> HMEEMIRSLQQ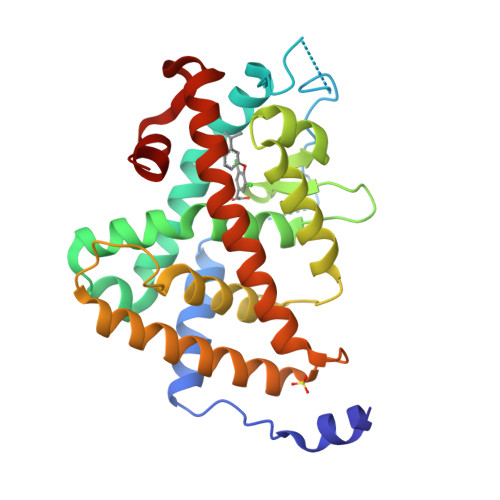RPEPTPEEWDLIHIATEAHRSTNAQGSHWKQRRKFLPDDIGQSPIVSMPDGDKVDLEAFSEFTKIITPAITRVVDFAKKLPMFSELPCEDQIILLKGCCMEIMSLRAAVRYDPESDTLTLSGEMAVKREQLKNGGLGVVSDAIFELGKSLSAFNLDDTEVALLQAVLLMSTDRSGLLCVDKIEKSQEAYLLAFEHYVNHRKHNIPHFWPKLLMKVTDLRMIGACHASRFLHMKVECPTELFPPLFLEVFEDQ> GSELQPPEASIAVVSIPRQLPGSHSEAGVQGLSAGDDSELGSHCVAQTGLELLASGDPLPSASQNAEMIETGSDCVTQAGLQLLASSDPPALASKNAEVTGTMSQDTEVDMKEVELNELEPEKQPMNAASGAAMSLAGAEKNGLVKIKVAEDEAEAAAAAKFTGLSKEELLKVAGSPGWVRTRWALLLLFWLGWLGMLAGAVVIIVRAPRCRELPAQKWWHTGALYRIGDLQAFQGHGAGNLAGLKGRLDYLSSLKVKGLVLGPIHKNQKDDVAQTDLLQIDPNFGSKEDFDSLLQSAKKKSIRVILDLTPNYRGENSWFSTQVDTVATKVKDALEFWLQAGVDGFQVRDIENLKDASSFLAEWQNITKGFSEDRLLIAGTNSSDLQQILSLLESNKDLLLTSSYLSDSGSTGEHTKSLVTQYLNATGNRWCSWSLSQARLLTSFLPAQLLRLYQLMLFTLPGTPVFSYGDEIGLDAAALPGQPMEAPVMLWDESSFPDIPGAVSANMTVKGQSEDPGSLLSLFRRLSDQRSKERSLLHGDFHAFSAGPGLFSYIRHWDQNERFLVVLNFGDVGLSAGLQASDLPASASLPAKADLLLSTQPGREEGSPLELERLKLEPHEGLLLRFPYAA;> MVRKPVVSTISKGGYLQGNVNGRLPSLGSKEPPGQEKVQLKREITLLDGVSLIVGTIIGAGIFVSPKGVLKNTGSVGLSLVIWAVCGVLSLFGALCYAELGTTIPKSGGAYLYILETFGPLPAFLRGWNELLIIRPASTAVISLAFGNYILEPFFPTCEPPELAIKLLAAVGILLLTVLNSLSVKWSARVQDFFTAAKLLALLIIIVPGVVQLIKGQTQNFKDAFEGSDPSIGGLPLAFYSGLYAYVGWDYLNFVTEEVKNPEKNIPLAIVISMPIVTVAYVLTNVAYFTTLSPEELLLSNAVAVTFGERLLGNFSWAVPIFVALSCFGSLNGSLFAMSRLFYVAAREGHLPKILSMIHVRRHTPLPALIVSGPLTAIMLFLGDLFSLINFMSFGTWLFYGLVVAGLIYLRYKKPDLHRPIKVPLFIPILFLLTCLFLVAVSLYSDPVNCGIGFVIILTGVPVYFLFVYWDKKPKWFRRISEKITRHLQLLLEVVPEEDKLDYKDDDDK

Among them, the heteromeric amino acid transporters (HATs) are unique members composed of two subunits, the light chain (SLC7) and the heavy chain (SLC3), linked by a conserved disulfide bridge. The light chain consists of 12 transmembrane helices and belongs to the amino acid‐polyamine‐organocation transporter (APC) superfamily. − amino‐acid transporter (SLC7A11, also named xCT) is a Na+‐independent electroneutral exchange system for cystine/glutamate.

As wild‐type xCT‐CD98hc displayed poor stability and could not be purified to homogeneity, we applied a consensus mutagenesis approach to xCT. The consensus mutated construct exhibited increased stability as compared to the wild‐type, and enabled the cryoelectron microscopy (cryo‐EM) map to be obtained at 6.2 Å resolution by single‐particle analysis. The N‐terminal transmembrane domain of CD98hc is adjacent to the TMD of xCTcons, consistent with the previous cryo‐EM model. TM1 and TM6 are apart from the substrate translocation pathway and create the cytoplasmic open cavity, similar to those in LAT1 structures, indicating that our structure captures an inward‐open state of xCTcons. The substrate‐binding pocket is also located at the same position as that of LAT1 and is empty, consistent with the absence of a substrate in our sample preparation. The ten TMs represent the common architecture of the APC superfamily consisting of three subdomains, hash, bundle, and arms. The cryo‐EM densities of the hash domain, characterized by the four helices arranged as a ‘hash’ character, are clearly resolved [Figure 5(a)]. The indistinct electron density suggests the structural flexibility of this domain. Notably, the current cryo‐EM density clearly showed the existence of a C‐terminal helix running parallel to the membrane, which was not visible in our previous structure of LAT1‐CD98hc, but detected in another study [Figure 3(a), 3(b)]. In the current case, xCTcons contains mutations of 20.2% residues over the whole protein, including the putative substrate binding pocket. Although wild‐type xCT shows Na+‐independent glutamate transport activity, xCTcons has lost this activity.> HMGSAPGQKECDNALRQLETVRELLENPVQPINDMSYFG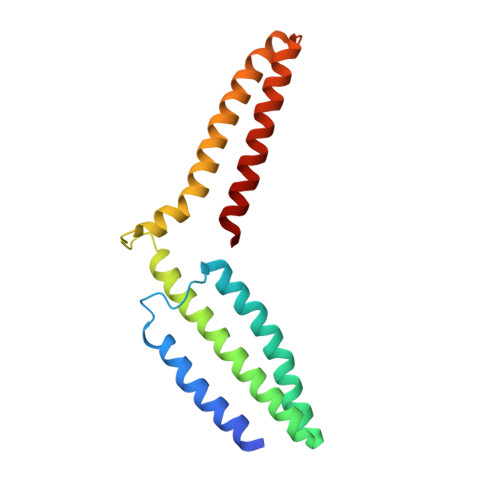CLDSVMENSKVLGEAMTGISQNAKNGNLPEFGDAIATASKALCGFTEAAAQAAYLVGVSDPNSQAQISPEGRAAMEPIVISAKTMLESAGGLIQTARALAVNPRDPPRWSVLAGHSRTVSDSIKKLITSMRD>[2x]MAEDPDPTEYLYISMEQKRKDQTKPYDGKKMVWVADEKEGYLLGLIKSTQGDICTVDIEGQESRQVKKDLLQQVNPPKYEKCEDMSNLTYLNDASVLHNLKQRYYANLIYTYSGLFCVAINPYKRFPIYTNRTVQIYKGRRRTEVPPHLFAISDGAYSAMLANRENQSMLITGESGAGKTENTKKVIAYYANVGAATPKPGKEAPTKEKKATLEDQVVQTNPVLEAFGNAKTVRNDNSSRFGKFIRIHFGPMGKLAGADIETYLLEKARVISQQTLERSYHIFYQLMSGGIENLKADLLLSDDIYDYHFVSQGKIEIPGVDDAEELRLTDTAFDILGFSHEYKTDVYKITASCMHLGEMKFKQRPREEQAEADGTEEGERVAHLLGVNAADLYKNLVKPKIKVGNEMVTQGRNATQVSYSVGGLAKAMFDRTFKWLVKRLNETLDTKQKRQYFIGVLDIAGFEIFDYNGFEQLCINFTNEKLQQFFNHHMFVLEQEEYKREGIDWVFIDFGLDLAACIELIEKPMGILSILEEESMFPKATDKSFQDKLNANHLGKSPNFVKPKPPKPGQQEAHFSIAHYAGTVPYNITGWLEKNKDPVNDTVVDQFKKGSNKLVQEIFEDHPGLGAEEKGGGGKGGGGRKKGASFQTVSALYREQLNRLMASLHSTQPHFVRCIIPNELKQPGVIDSGLVMHQLTCNGVLEGIRICRKGFPNRMVYPDFKQRYTILAASAVPKGFVDAKKVTEAVLGAIQLDANDYRLGNTKVFFRAGVLGRLEEMRDDRLGKIVTWLQAWIRWYLSKKEFKKLQEQRVALLVIQRNLRKFLTLRNWLWYKLYIKVKPLLTMAKVEDELKALEEKLKKALESLEKEEKVRKDIEVQNVKLLQEKNDLFLQLESERSGAGDVEERLTKAISMKNDLEGQVQELQERLSREEDAHSNLSSVRKKLDGEISNLKKEIEDLQLVIQKTEQDKAAKDHQIRNLNDEIAHQDELINKLNREKKQMQEMGQKTGEDLQATEDKLNHMNKVKAKLEQTLDELEDSLEREKKLRGDVEKTKRKVEGDLKLAQEAVADLEKNKKELEQALQRKEKEMASLSAKLEDEQGLVAKLQKQIKELQARIEELEEELEAERQARAKAEKQRADLAREIEELSERLEEAGGATSAQVELNKRREAEMAKLRRDLEESNIQHEQTLANLRKKHNDVVAELSEQIDQLNKHKARLEKEKAQMKGELDDVRSSVDHVNKEKANAEKQAKQLEMQLTELQGKMDEAHRSLGDFDAAKKRLTVENTELTRQLEDAESQVSQLSKLKTSLQTQLEDTKRMADEESRERATAMGKFRSVEHDLDSLREQIDEEQEGKADLQRQLSKANAEVQLWRSKYESEGLARLEELEESKRKLDAKLQEAMETIDQLNSKTSGLEKTKSRLQGELEDMTIEVEKANALASAMEKKQKSFDRIISEWKQKVDDLALELDASQKECRNYSTEVFKLRSQYEESQEHYESVKRENKNLQDEIKDLVDQLGEGGRSVHELEKARKRLELEKEELQAALEEAEAALEQEENKVLRAQLELSQVRQ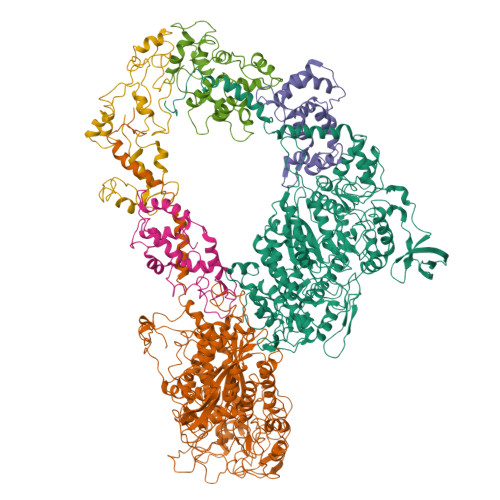EIDRRLQEKEEEFENTRKNHQRAIDSMQASLEAEAKGKAEALRMKKKLESDINELEIALDHSNKANAEAQKNIKKYQIQLKETQQALEEEQRARDEVREQYAMSERRCNAMHGELEESRQLLEQADRARRAADSELAELHENVNELSAQNSSLSMAKRKLEGEMQALHADLDEMLNEAKSSEEKAKKAMVDAARLADELRAEQEHAQQQEKMRKAMEGQIKELQVRLDEAEAAALKGGKKIIQKLEQKVRELETELDNEQRRHSEAAKNVRRSERRVKELQFQAEEDRKNQERMQDLVDKLQQKIKTYKRQIEEAEEIAALNLAKFRKVQQELEDAEERADMAENVAAKLRAKNRSSASVGRAMSPIPMGKPGRPKSKIDEE;>[2x]MADLKAAEVEKAREHFEIYDWEGEGKIDARDLGDLLRSLDCKPTLAMVKKNGGSDKRGEKKLTLEEFLPIFSQIKKEKEVGTLEDFMEGLKVYDKAENGTMLAAELAHVLLSLGERLTDIECEEIMRVCDEDDDGFLKYEPFVKTIIAGPFPDEGK;>[2x]MGDEEKKEKKKKSKKKSEEEGGDAAPAPPPPKPPSQKRRAQRSGSNVFAMFTQHQVQEFKEAFQLIDQDKDGFISKNDIRATFDSLGRLCTEQELDSMVAEAPGPINFTMFLTIFGDRIAGTDEEDVIVNAFNLFDEGEGKCKEETLKRSLTTWGEKFSQDEVEEALSEAPIDGNGLIDIKKFAQILTKGAEEEGA>[2x]MVLYFIGLGLYDERDITVKGLEIAKKCDYVFAEFYTSLMAGTTLGRIQ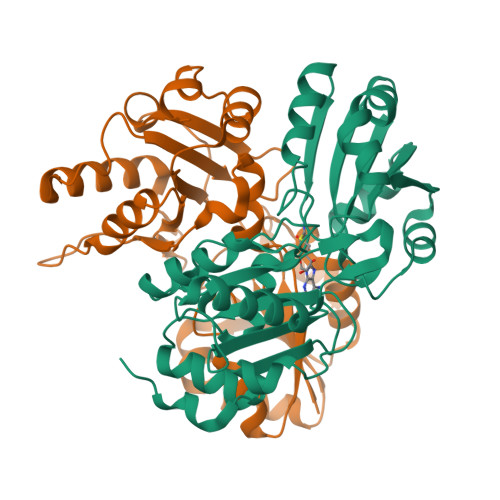KLIGKEIRVLSREDVELNFENIVLPLAKENDVAFLTPGDPLVATTHAELRIRAKRAGVESYVIHAPSIYSAVGITGLHIYKFGKSMTVAYPEGNWFPTSYYDVIKENAERGLHTLLFLDIKAEKRMYMTANEAMELLLKVEDMKKGGVFTDDTLVVVLARAGSLNPTIRAGYVKDLIREDFGDPPHILIVPGKLHIVEAEYLVEIAGAPREILRVNV> GSHEMIKSLQHRPSPSAEEWELIHVVTEAHRSTNAQGSHWKQKRKFLPEDIGQSPMASMPDGDKVDLEAFSEFTKIITPAITRVVDFAKKLPMFSELPCEDQIILLKGCCMEIMSLRAAVRYDPESETLTLSGEMAV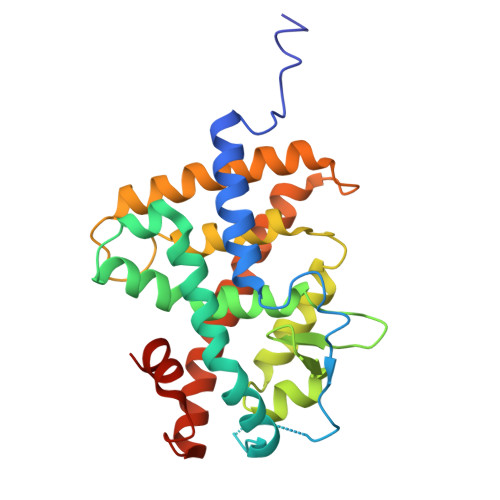KREQLKNGGLGVVSDAIFDLGKSLSAFNLDDTEVALLQAVLLMSSDRTGLICVDKIEKCQETYLLAFEHYINYRKHNIPHFWPKLLMKVTDLRMIGACHASRFLHMKVECPTELFPPLFLEVFEDQEV>[2x]SAPRIMRLVAECSRSRARAGELWLPHGTVATPVFMPVGTQATMKGITTEQLDALGCRICLGNTYHLGLRPGPELIQKANGLHGFMNWPHNLLTDSGGFQMVSLVSLSEVTEEGVRFRSPYDGNETLLSPEKSVQIQNALGSDIIMQLDDVVSSTVTGPRVEEAMYRSIRWLDRCIAAHQRPDKQNLFAIIQGGLDADLRATCLEEMTKRDVPGFAIGGLSGGESKSQFWRM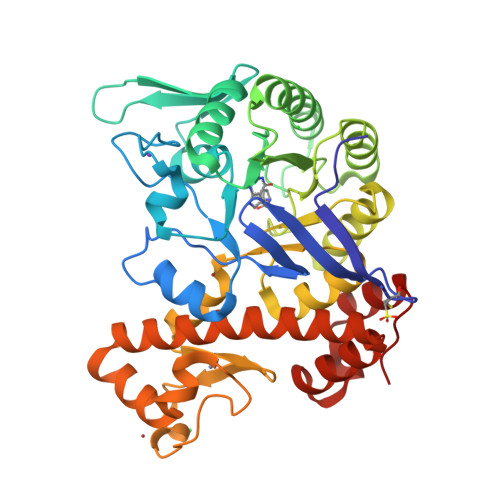VALSTSRLPKDKPRYLMGVGYATDLVVCVALGCDMFDCVFPTRTARFGSALVPTGNLQLRKKVFEKDFGPIDPECTCPTCQKHSRAFLHALLHSDNTAALHHLTVHNIAYQLQLMSAVRTSIVEKRFPDFVRDFMGAMYGDPTLCPTWATDALASVGITLG> Q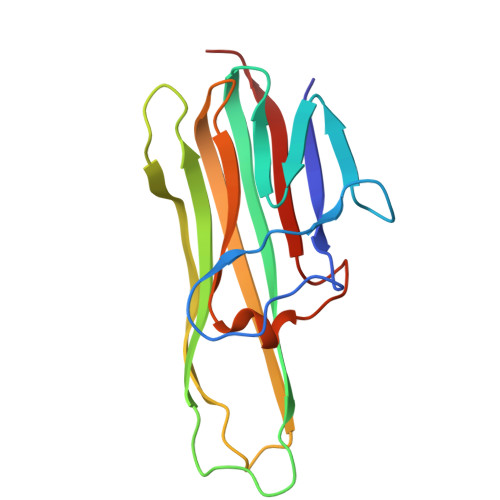PFAHLTINAASIPSGSHKVTLSSWYHDRGWAKISNMTLSNGKLRVNQDGFYYLYANICFRHHETSGSVPTDYLQLMVYVVKTSIKIPSSHNLMKGGSTKNWSGNSEFHFYSINVGGFFKLRAGEEISIQVSNPSLLDPDQDATYFGAFKVQDID The Tn1549 conjugative transposon propagates resistance to the antibiotic vancomycin used for severe drug-resistant infections. The DNA cleavage and joining reactions required for CTn transposition are carried out by a transposase enzyme called integrase (Int). Most known CTns, including the Tn916-like family, have Y-transposases that use a conserved tyrosine residue to attack a phosphorous atom in the DNA backbone. Int contains 3 functional domains: an arm-binding domain (AB), a core DNA binding domain (CB), and a catalytic domain (CAT).

To understand how Int can accommodate different CIs, we determined the structure of two additional Int82N-CI complexes. DNA sequences contained IRL and IRR sites connected by 6 bp homoduplex crossover regions of different sequence (CI6a and CI6b) (Lambertsen et al., 2018). The two Int82N-CI6 structures were solved at 2.7 Å resolution and show a similar architecture to the CI5 complex with two protein subunits binding one CI DNA. In both Int82N-CI6 complexes, the DNA assumes a similar conformation as in the CI5 complex. In the Int82N-CI6 complexes, one subunit is shifted with the CAT domains ∼2–3 Å further apart than in the Int82N-CI5 complex, reflecting small flexibility within the dimer. One difference is in the small loop after the β-hairpin, which shows an additional conformation in the CI6 structures located near the DNA crossover region. The maps at the crossover region in the CI6 structures are particularly poorly defined, suggesting that flexibility in this region helps accommodate CIs with different crossover lengths. Our two CI6 structures also show that different CI sequences can be accommodated in the center of the Int dimer similarly, again due to the distortions and flexibility of the crossover region.

>SMTVCQLYAKQIRHRGNVKHNTKLGRERLMRILEQDRLGSCPIDSVKLSDAKEWALRMKEKGLSYKTINNDKRSLKAAFYTAIQDDCIRKNPFDFQLSDVLDDDTEPKVPLTPAQEESFLSFIQGDKVYQKHYDAIVILLGTGLKISELCGLTDKDLDFENRVIIVSHQLLRNTGVGYYIDEPKTQSGVRKIPMNEEVYQAFQRVIKNRKGAKPFIIDGYANFLFLKQNGYPMTAVDYGGMFGRLVKKYNKSHEEALPKTTTPHAMRHTFCTRLANAGMNPKALQYIMGHSNITMTLNYYAHATFDSARAEMERLAA[2x]> WTPPRSPFNLVQETLFHDPWKLLIATIFLNRTSGKMAIPVLWKFLEKYPSAEVARTADWRDVSELLKPLGLYDLRAKTIV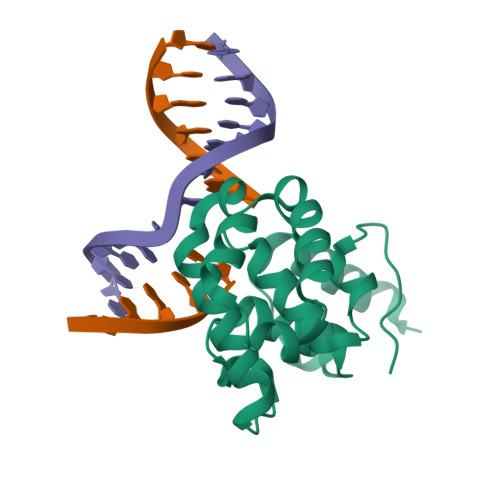KFSDEYLTKQWKYPIELHGIGKYGNDSYRIFCVNEWKQVHPEDHKLNKYHDWLWENHE> SIYNSFYVYCKGPCQRVQPGKLRVQCSTCRQATLTLTQGPSCWDDVLIPNRMSGECQSPHCPGTSAEFFFKCGAHPTSDKETSVALHLIATNSRNITCITCTDVRSPVLVFQCNSRHVICLDCFHLYCVTRLNDRQFVHDPQLGYSLPCVAGCPNSLIKELHHFRILGEEQYNRYQQYGAEECVLQMGGVLCPRPGCGAGLLPEPDCRKVTCEGGNGLGCGFAFCRECKEAYHEGECSAVFENLYFQSQAYRVDERAAEQARWEAASKETIKKTTKPCPRCHVPVEKNGGCMHMKCPQPQCRLEWCWNCGCEWNRVCMGDHWFDV

Parkin is an auto-inhibited ubiquitin E3 ligase activated by dual phosphorylation of its ubiquitin-like (Ubl) domain and ubiquitin by the PINK1 kinase. Parkin is an autoinhibited RBR family E3 ubiquitin ligase consisting of an N-terminal ubiquitin-like (Ubl) domain followed by four Zn2+ binding domains RING0, RING1, in-between-RING (IBR), and RING2. Like other RBR-family E3 ligases, Parkin binds to an E2, and ubiquitin is transferred from E2 onto the catalytic C431 residue (on RING2) of Parkin before ubiquitination of lysines on target substrates. Furthermore, C431 on RING2 is occluded by the RING0 domain of Parkin, which inhibits Parkin activity.

Further, to confirm that untethering does not affect the native interactions between RING2 and RING0 domains, we purified and determined the structure of untethered R0RBR (TEV) Parkin. Co-elution of R0RB (141-382) and RING2 (383-465) fragments on SEC and crystal structure analysis showing intact native interactions between RING2 and RING0 excluded the possibility of an artifact.>[4x]GP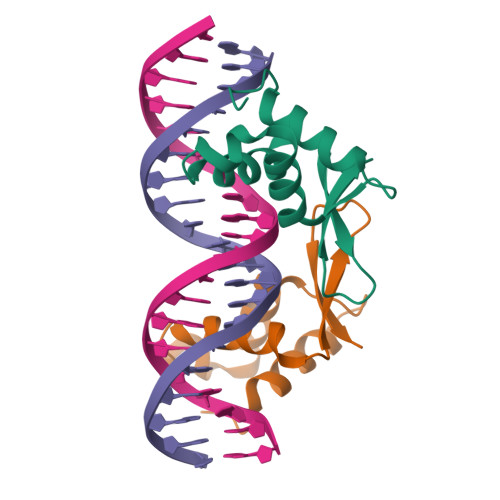SRPSASWQNSVSERPPYSYMAMIQFAINSTERKRMTLKDIYTWIEDHFPYFKHIAKPGWKNSIRHNLSLHDMFVRETSANGKVSFWTIHPSANRYLTLDQVFKPLDPGSPQLPEH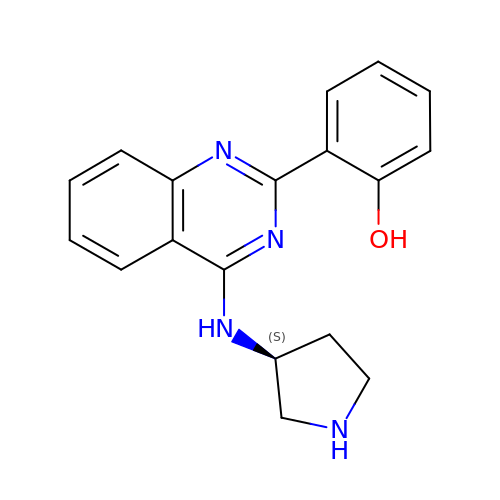2-{4-[(3S)-PYRROLIDIN-3-YLAMINO]QUINAZOLIN-2-YL}PHENOL | C18 H18 N4 O | XVURFLCQTYKQLW-LBPRGKRZSA-N>SEFMTEPAIITNASDPAVQRIIDVTKHSRASIKTTLIEDTEPLMECIRAGVQFIEVYGSSGTPLDPALLDLCRQREIPVRLIDVSIVNQLFKAERKAKVFGIARVPRPARLADIAERGGDVVVLDGVKIVGNIGAIVRTSLALGAAGIVLVDSDLATIADRRLLRASRGYVFSLPVVLADREEAVSFLRDNDIALMVLDTDGDLGVKDLGDRADRMALVFGSEKGGPSGLFQEASAGTVS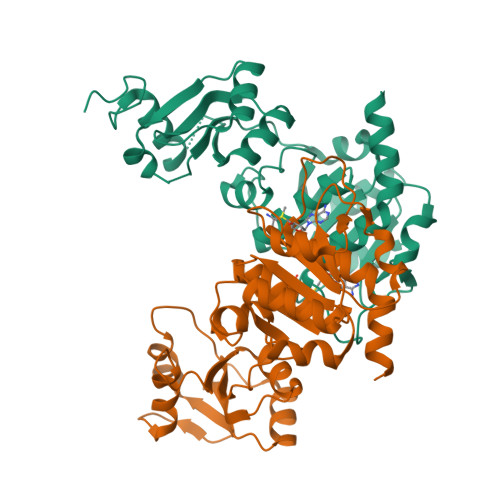IPMLSSTESLNVSVSVGIALHERSARNFAVRRAAAQA[2x]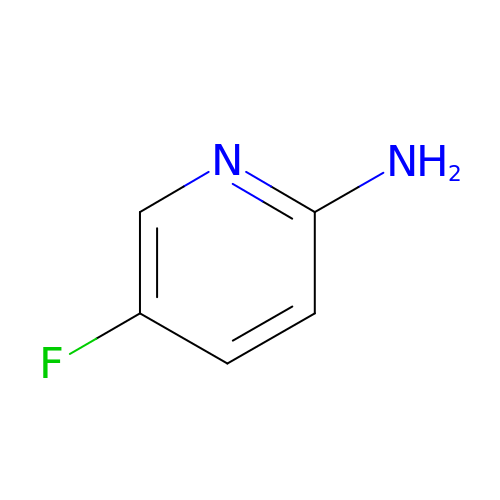5-fluoranylpyridin-2-amine | C5 H5 F N2 | YJTXQLYMECWULH-UHFFFAOYSA-N>[8x]GSDLP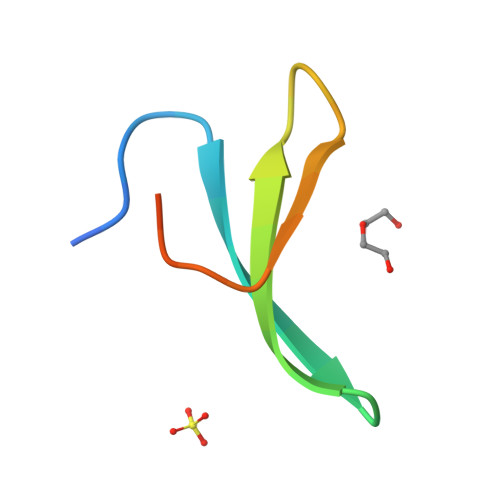AGWMRVQDTSGTYYWHIPTGTTQWEPPGRASPS> MYFQIRGIILWPRNKNFKPHTIRFELGKVNVISGASRTGKSAVIPIIDYCLGANTCSIPVKTIRKYCEWFGIVVATEQGEKLLARKEPGNQRSTTDMFVLEAENITSIPIRLEKNTNVIAVKRMLDDLANLSNLDFSGGDENSGFDGRPAFRDLAAFTFQPQNVVANPDVLFFKTNTYEHREKLRKIFPYVLGAITSELMAKQFELNRIRLFLRRKERELKDAQDVSAQWLADLKSKYSEAQELGLVPK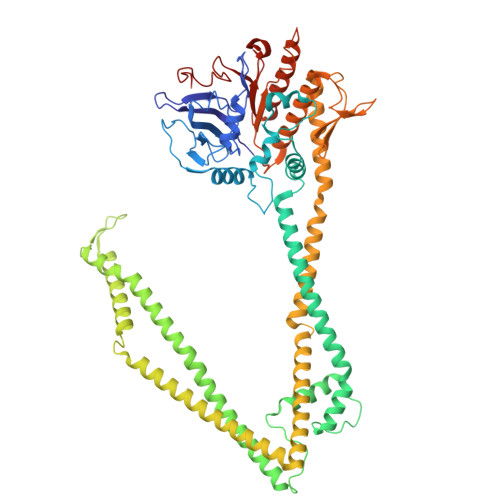PQEQLSRKQMISQLEEVISRTDLTLKVTVSTISDALSELNTLESEERLVSRELTTMRHRLEEMNRLRVGMHQYENALLMQRDRLKISGWLLSNTNDESDCPMCGSHTDSAKQKLQALVQRLSDVEAAVGADAHKEVPAAFDRELQRVTTEVANATERLRAIQSRKRTLTSRSKEAREQQFSTRRAERFIGNVESALELHRKLGSDSELVEEVRKLKEMVQTLEKELREKDVELRKNQALRVINAQAGNILQGLDVEDPSAPISLEINDLTIKVLGDERDDYLSEIGSGSNWLSYHLAILLSLHQFYLSQKNNPVPSFLILDQPSQVYFPKTTQLPNIANEDEPKLRDEDVEAVRRAFKAMGNVVIKEKGKLQLIVLDHAPREVWGEIDGVVGLPEWRDGIKLVPMEWLTGV> XSYIDKIADLIRKVAEEI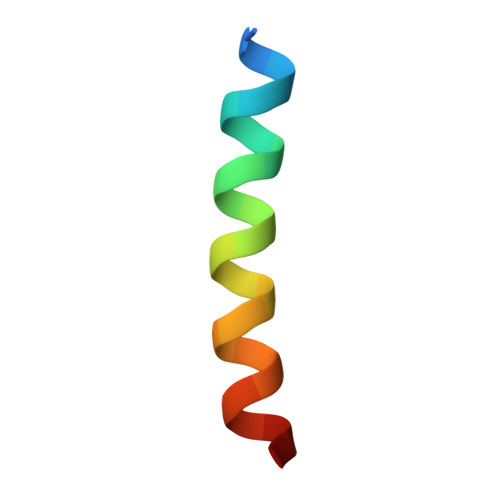NSKLEX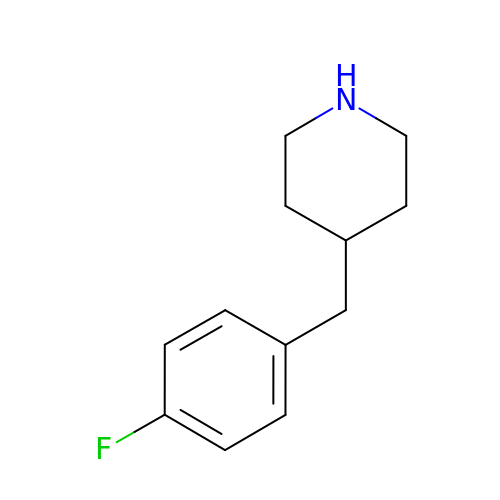4-(4-FLUOROBENZYL)PIPERIDINE | C12 H16 F N | JLAKCHGEEBPDQI-UHFFFAOYSA-N> NPVENYIDSVLNEVLVVPNIQPSTSVSSHAAPALDAAETGHTSSVQPEDMIETRYVITDQTRDETSIESFLGRSGCIAMIEFNTSSDKTEHDKIGKGFKTWKVSLQEMAQIRRKYELFTYTRFDSEITIVTAA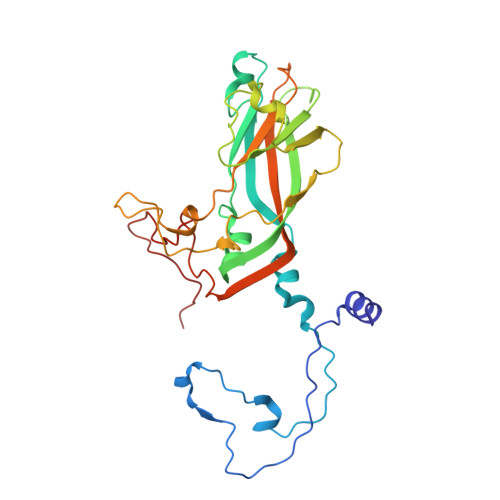AAQGNDSGHIVLQFMYVPPGAPVPEKRDDYTWQSGTNASVFWQEGQPYPRFTIPFMSIASAYYMFYDGYDGDSAASKYGSVVTNDMGTICVRIVTSNQKHDSNIVCRIYHKAKHIKAWCPRPPRAVAYQHTHSTNYIPSNGEATTQIKTRPD> DLDL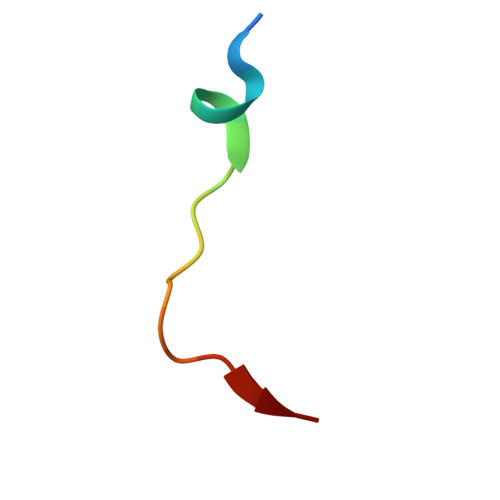EMLAPYIPMDDDFQL> G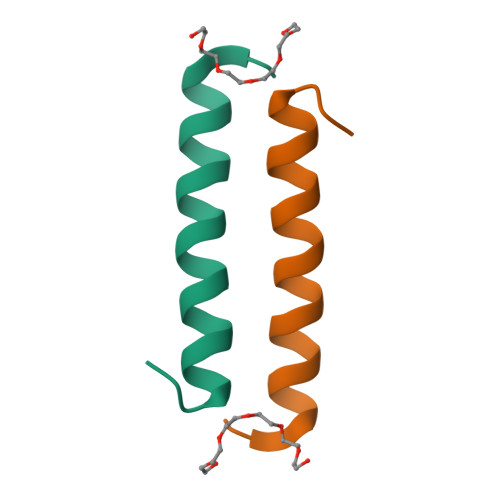GSLTEQDRQLRLLQAQIQRLLEAQSLM>MAPRKFFVGGNWKMNGDKKSLGELIHTLNGAKLSADTEVVCGAPSIYLDFARQKLDAKIGVAAQNCYKVPKGAFTGEISPAMIKDIGAAWVILGHSERRHVFGESDELIGQKVAHALAEGLGVIACIGEKLD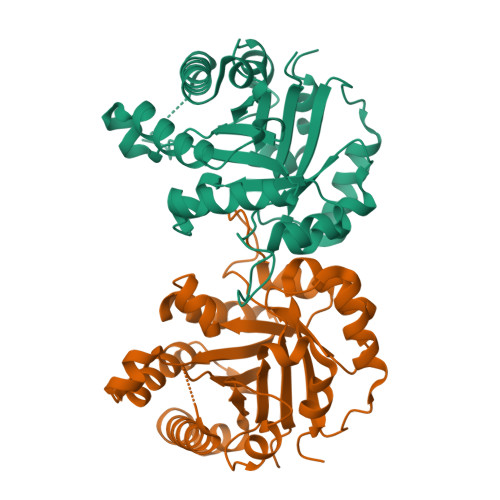EREAGITEKVVFEQTKAIADNVKDWSKVVLAYEPPEAIGTGKTATPQQAQEVHEKLRGWLKSHVSDAVAQSTRIIYGGSVTGGNCKELASQHDVDGFLVGGASLKPEFVDIINAKH[2x]(4-azanylpiperidin-1-yl)-cyclopropyl-methanone | C9 H16 N2 O 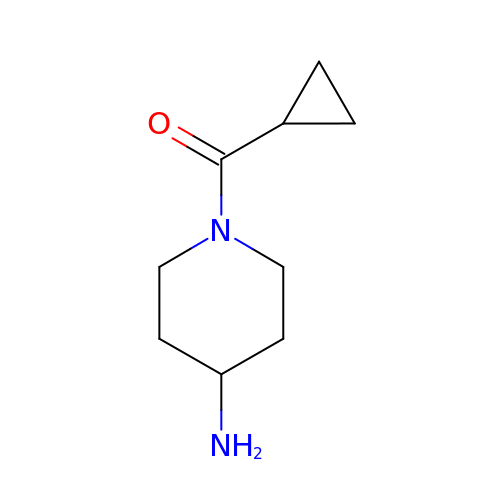| GCYSQXZPDQBVCH-UHFFFAOYSA-N> GIPGTTTPITKEMEPNDDIKEANGPIVEGVTVKGDLNGSDDADTFYFDVKEDGDVTIELPYSGSSNFTWLVYKEGDDQNHIASGIDKNNSKVGTFKSTKGRHYVFIYKHDSASNI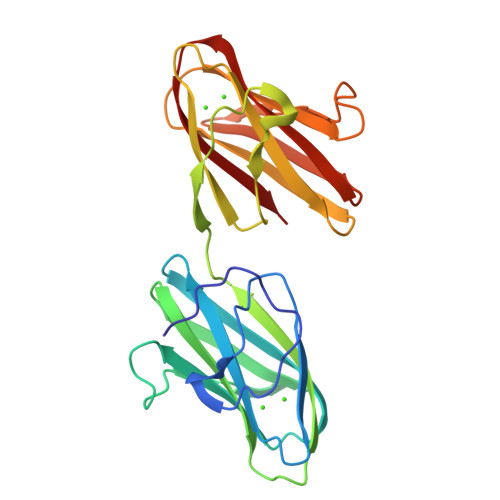SYSLNIKGLGNEKLKEKENNDSSDKATVIPNFNTTMQGSLLGDDSRDYYSFEVKEEGEVNIELDKKDEFGVTWTLHPESNINDRITYGQVDGNKVSNKVKLRPGKYYLLVYKYSGSGNYELRVNK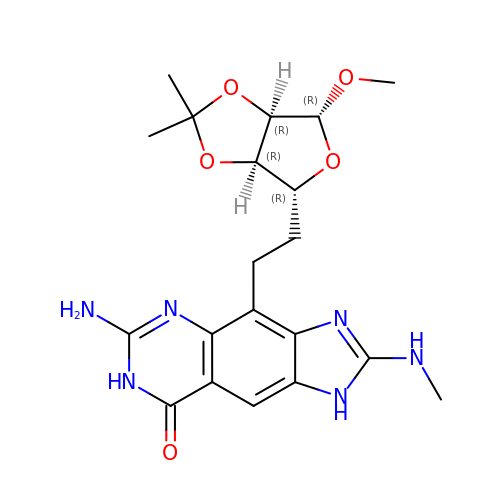4-[2-[(3~{a}~{R},4~{R},6~{R},6~{a}~{R})-4-methoxy-2,2-dimethyl-3~{a},4,6,6~{a}-tetrahydrofuro[3,4-d][1,3]dioxol-6-yl]ethyl]-6-azanyl-2-(methylamino)-1,7-dihydroimidazo[4,5-g]quinazolin-8-one | C20 H26 N6 O5 | VLKGVMAOHRTCMF-BNGXUDDSSA-N>[4x]TNMSIKEQRESLPVFQFRDQIIQAVKDNQILIVVGETGSGKTTQVTQYLAEAGFTKYGMIGCTQPRRVAAVSVAKRVAEEVGCQLGQEVGYTIRFEDVTSPATKIKYMTDGMLQREILMDPDLKRYSVIMLDEAHERTIATDVLFALLKKTVKRRPDLKVIVTSATLDAEKFSEYFNSCPIFTIPGRTFPVEILYSREPEPDYLEAALTTVMQIHLTEPPGDILVFLTGQEEIDTACEILYERMKALGPSVPELIILPIYSALPSEMQSRIFEPAPPGSRKVVIATNIAETAITIDYIYYVVDPGFVKQNAYDPKLGMDSLVVTPISQAQANQRAGRAGRTGPGKCFRLYTEAAYQSEMLPTTIPDIQRQNLANTILLLKAMGINDLLRFDFMDPPPVNTMLTALEELYALGALDDEGLLTRLGRKMADFPMEPSLSKVLIASVDKGCSDEMVTIVSMLNLQQIFYRPKDKQQQADQKKAKFHDPTGDHLTLLNVYNAWKNSGYSNAWCFENYIQARAMRRARDVRQQIVKIMERHRHPIISCGRDTDKIRQALCAGFFRNTARKDPQEGYKTLTEGTPVYLHPSSALFGKQAEWVLYHELVLTTKEYMHFTTAIEPKWLVEAAPTFFKLAPTDRLSKRKKAERIQPLYNKYEGEDGWRLSAQRRAARPGGGGGTWG

DEAH-box adenosine triphosphatases (ATPases) play a crucial role in the spliceosome-mediated excision of pre-mRNA introns. The catalytic activation, the catalysis itself as well as the final disassembly steps are driven by so-called DEAH-box helicases. They all belong to the helicase superfamily 2 (SF2) and share at least eight conserved sequence motifs (motifs I, Ia, Ib, II, III, IV, V and VI) spread over two RecA-like domains that together form the helicase core. Two RecA-like domains, referred to as RecA1 and RecA2, build up the helicase core. The RecA2 domain contains an anti-parallel β-hairpin present in all DExH-box helicases, which protrudes out of the RecA2 domain thereby contacting the C-terminal domains. These domains are divided in three distinct domains, namely the winged-helix (WH), the helix-bundle (HB) and the oligonucleotide-binding (OB) domain.

A structural analysis revealed that a serine in motif V is involved in polar interactions with one of the ligands in all structurally characterized catalytic states. In the adenosine nucleotide-free but RNA-bound state, the side chain of the serine contacts the U7 phosphate and thereby bridges the gap that is formed by the more distant conformation of the RecA-like domains. In order to verify the central role of this serine, we created alanine, glycine and proline mutants of this residue in Prp22 and characterized their ATPase activity. The lack of the hydroxyl group in Prp22-S837A mainly leads to an increase of kcat regardless of the presence of RNA and only to a minor decrease of Km when RNA is present. In both cases, the catalytic efficiency (kcat/Km) is improved by a factor of ∼1.7. We could furthermore structurally characterize Prp22-S837A in the adenosine nucleotide-free but RNA-bound state, as well as Prp43-S387A and Prp43-S387G in the ATP-bound state. The structures of these three mutants show that motif V is able to adopt the same nucleotide-specific conformations regardless of the side chain property. Summarizing our data show that the serine side chain is dispensable for the function of motif V and instead has a regulatory role. The polar interactions of the hydroxyl group with the RNA phosphate and active site components seem to negatively regulate the turnover rate of DEAH-box ATPases.>[2x]MTDNNNYRDVEIRAPRGNKLTAKSWLTEAPLRMLMNNLDPQVAENPKELVVYGGIGRAARNWECYDKIVETLTRLEDDETLLVQSGKPVGVFKTHSNAPRVLIANSNLVPHWANWEHFNELDAKGLAMYGQMTAGSWIYIGSQGIVQGTYETFVEAGRQHYGGSLKGKWVLTAGLGGMGGAQPLAATLAGACSLNIESQQSRIDFRLETRYVDEQATDLDDALVRIAKYTAEGKAISIALHGNAAEILPELVKRGVRPDMVTDQTSAHDPLNGYLPAGWTWEQYRDRAQTEPAAVVKAAKQSMAVHVQAMLDFQKQGVPTFDYGNNIRQMAKEEGVANAFDFPGFVPAYIRPLFCRGVGPFRWAALSGEAEDIYKTDAKVKELIPDDAHLHRWLDMARERISFQGLPARICWVGLGLRAKLGLAFNEMVRSGELSAPVVIGRDHLDSGSVSSPNRETEAMRDGSDAVSDWPLLNALLNTA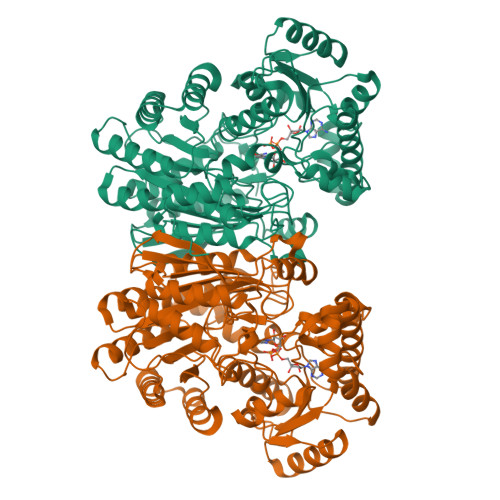GGATWVSLHHGGGVGMGFSQHSGMVIVCDGTDEAAERIARVLTNDPGTGVMRHADAGYDIAIDCAKEQGLDLPMITG> GPLGSPEFMNKQWYLLANQLILSLSKYEGGHIFEKLVDAKKQNCPDYYDVIKNPMSFSCIKTKLKKGQYAYPSEFVKDVQLIFDNCSLYNTSNSVVAITGKNIETYFNNQLIVMGYNNFILKEKKINDMLKLVEEEN

In this study, the focus is on the essential Bromodomain protein 1 (PfBDP1) of the malaria pathogen Plasmodium falciparum. Possible targets are the nine predicted bromodomain (BRD) proteins, among which PfBDP1 has been identified as essential in the blood stage of P. falciparum. PfBDP1 is involved in regulating erythrocyte invasion genes and conditional knockdown (KD) of PfBDP1 lead to a significantly reduced multiplication rate during the intraerythrocytic development cycle (IDC). PfBDP1 is recruited to promoters of invasion‐related genes by binding with its BRD to acetylated histones.

BP and BM are very similar to PfBDP1‐BRD‐RMM2, with most of the methyl group orientated the same way but also with a much smaller proportion rotated by 180°. The amide does not appear to interact directly with the BP in the crystal, but this does not have to be the case in solution. Notably, His354 forms a hydrogen bond to a symmetry equivalent and may be no longer available. Based on the two conformations of RMM23 in the PfBDP1‐BRD co‐crystal structure, this should be possible for RMM23 and RMM22, but not for RMM21 (compared to RMM20). Treatment of synchronous ring‐stage 3D7 and NF54 parasite cultures with RMM23 resulted in significantly reduced growth after 48 h of treatment, indicating that the compound blocked parasite development within the same IDC when treatment was initiated. The conditional KD parasites (10 nM Shld1) exhibited increased sensitivity against RMM23, which was reflected by a leftward shift in the dose–response curve compared to standard conditions (500 nM Shld1). In contrast, the EC50 of chloroquine was unchanged. This observation is consistent with RMM23 acting directly on PfBDP1. To examine whether RMM23 inhibits chromatin binding of PfBDP1‐BRD, we performed ChIP of PfBDP1HA in schizont stage parasites cultivated for 3 h with 50 μM RMM23 or DMSO control. Analysis of several known PfBDP1 target loci by qPCR revealed significantly diminished enrichment of PfBDP1 in the presence of RMM23, further supporting PfBDP1‐BRD as the main target of RMM23 in P. falciparum parasites. Using in vitro assays combined with conditional KD of PfBDP1, we identified RMM23 as a PfBDP1‐specific inhibitor that demonstrated effective binding and inhibition of parasite growth.> RDPTLTLSLIAKNTPANSMIMTKLPSVRVKTEGYNPSIN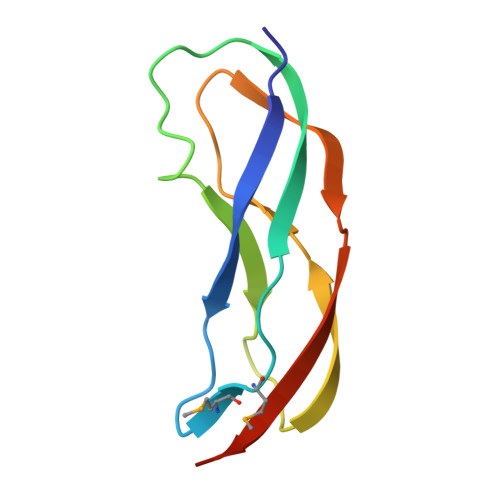VNELFAYVDLSGSEPGEHDYEVKVEPIPNIKIVEISPRVVTLQLEHHHHHH> RQNLQMEIKITTVIQHVFQNLILGSKVNWAEDPALKEIVLQLEKNVDMM;> MDALQMAVGYFEKGPIKASQNKDKTLEKHLKTVENVAWKNGLASEEIDILLNIALSGKFGNAVNTRILKCMIPATVISEDSVVKAVSWLCVGKCSGSTKVLFYRWLVAMFDFIDRKEQINLLYGFFFASLQDDALCPYVCHLLYLLTKKENVKPFRVRKLLDLQAKMGMQPHLQALLSLYKFFAPALISVSLPVRKKIYFKNSENLWKTALLAVKQRNRSPLEVQFG;> KMLNIKEYKEKLLSTLGEFLEDHFPLPDRSVKKKKKNIQESSVNLITLHEMLEILINR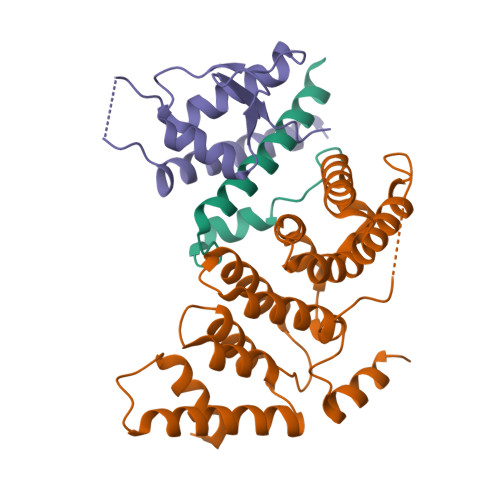LFDVPHDPYVKISDSFWPPYVELLLRNGIALRHPEDPTRIRLEAFHQ(3R,3'R)-3-anilino-1'-(7H-pyrrolo[2,3-d]pyrimidin-4-yl)[1,3'-bipiperidin]-2-one 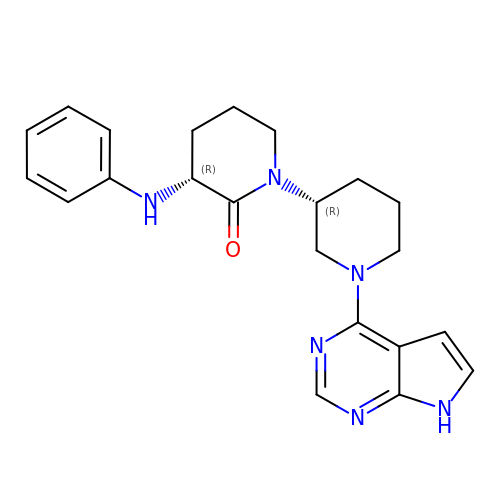| C22 H26 N6 O | BYRYLAFNCJLOIQ-IEBWSBKVSA-N> QDEVLSEAFRLTITRKDIQTLNHLNWLNDEIINFYMNMLMERSKEKGLPSVHAFNTFFFTKLKTAGYQAVKRWTKKVDVFSVDILLVPIHLGVHWCLAVVDFRKKNITYYDSMGGINNEACRILLQYLKQESIDKKRKEFDTNGWQLFSKKSQEIPQQMNGSDSGMFACKYADCITKDRPINFTQQHMPYFRKRMVWEI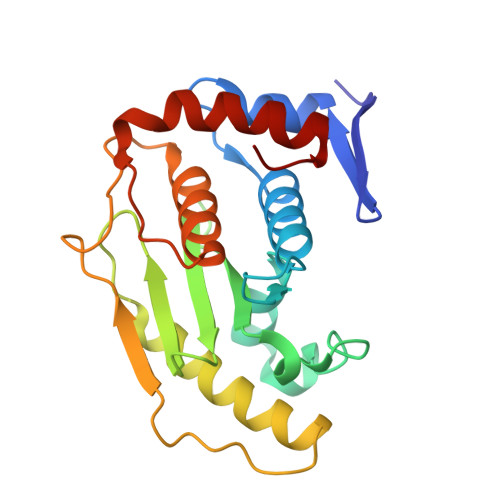LHRKLL> GKSASGIIMETQQAKQTLADIEARHADIMKLETSIRELHDMFMDMAMLVESQGEMIDRIEYNVEAAVDYIETAK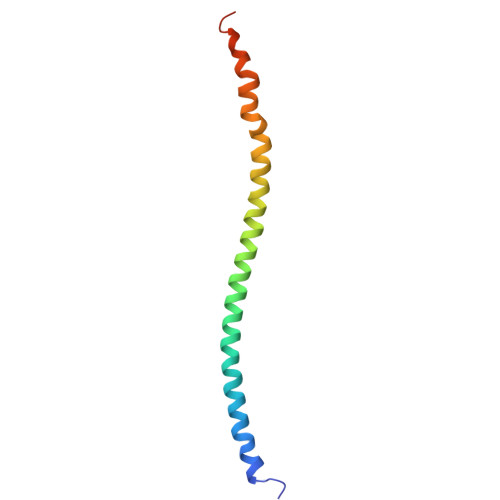VDTKKAVKYQSKAR>MGSSHHHHHHSSGRENLYFQGVEYGFWLPIFGGWLRNVNDESMPPTFEYAKQTAQAAEQLGFSTTLIAELNLNDIKGVSAPSLEAWTTAAALAAVTDRLEIMTAVRPGFHNPAVTAKMAANIDQLSNGRFTLNVVSAWWEEEAKQYGGVFTAHDERYDRTEEFVTILKGLWKEEEFSYKGNFYELHHTHLSPKPVQKQGIKLYAGGESKRGKEVIVNHADAYVMHGGTVEEVSVKIEDMKNRRKKVTEEPLQSFGLAAYVICRHTEEEALEEWRRITDVKDDALGYAGYQDFVSKSQLEQQVKLNDYSVSNRGLRPNLIGTPEQIAERILAFEKVGVTLLLLQFSPQLEEMKR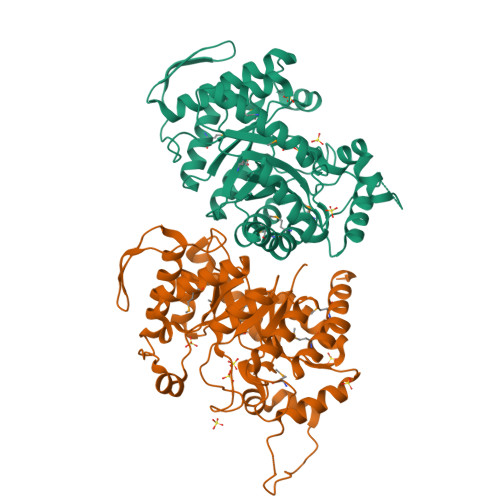FSEKVMPLVEAKRKELIT[2x]6-(2H-indazol-4-yl)-1-methyl-N-[3-(methylsulfonyl)propyl]-1H-pyrazolo[3,4-d]pyrimidin-4-amine 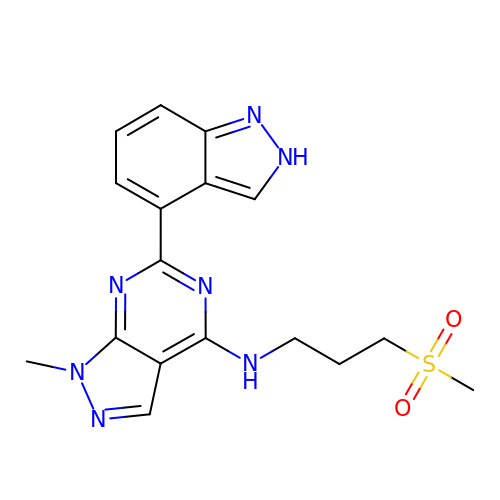| C17 H19 N7 O2 S | YZTXAMRYFBNCHP-UHFFFAOYSA-N> MAEPVSPLKHFVLAKKAITAIFDQLLEFVTEGSHFVEATYKNPELDRIATEDDLVEMQGYKDKLSIIGEVLSRRHMKVAFFGRTSSGASSVINAMLWDKVLPSGIGHITNCFLSVEGTDGDKAYLMTEGSDEKKSVKTVNQLAHALHMDKDLKAGCLVRVFWPKAKCALLRDDLVLVDSPGTDVTTELDSWIDKFCLDADVFVLVANSESTLMNTEKHFFHKVNERLSKPNIFILNNRWDASASEPEYMEDVRRQHMERCLHFLVEELKVVNALEAQNRIFFVSAKEVLSARKQKAQGMPESGVALAEGFHARLQEFQNFEQIFEECISQSAVKTKFEQHTIRAKQILA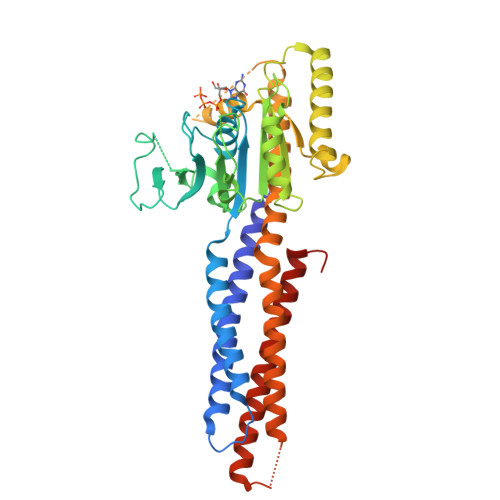TVKNIMDSVNLAAEDGSGSGSGGSEIARLPKEIDQLEKIQNNSKLLRNKAVQLENELENFTKQFLPSSNEES> GSHMEEDWIREYPPITSDQQRQLYKRNFDTGLQEYKSLQSELDEINKELSRLDKELDDYREESEEYMAAADEYN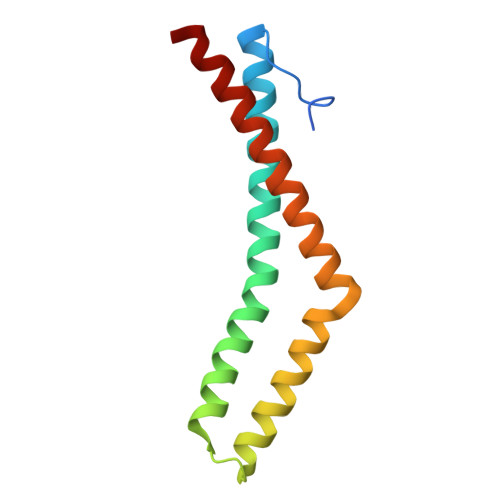RLKQVKGSADYKSKKNHCKQLKSKLSHIKKMVGDYDRQKT CysZ family members are 28–30 kDa bacterial inner-membrane proteins found exclusively in prokaryotes with no apparent homology to any of the established channel or transporter folds, and are scarcely studied in the literature. The CysZ protomer is an alpha-helical integral membrane protein with two long transmembrane (TM) helices (H2b and H3a) and two pairs of shorter helices (H4b-H5a and H7-H8) that insert only partially into the membrane (hemi-penetrating), forming a funnel or tripod-like shape within the membrane. The protein has an extra-membranous hydrophilic ‘head’, comprising an iris-like arrangement of the two short helices, H1 and H6, and kinked helices H3b, H4a, and H5b. Besides not resembling other transporter structures, CysZ mediates sulfate flux into cells or proteoliposomes without coupling to ion gradients, partner proteins, or exogenous energy sources such as ATP.

The structure of PfCysZ was solved second, to 3.5 Å resolution, with crystals also belonging to space group C2. Although PfCysZ and IlCysZ share 42% sequence identity, molecular replacement failed to find a convincing solution, and we instead used SeMet-derivatized PfCysZ to obtain phase information by multi-crystal SeMet SAD. Unlike PdCysZ, both IlCysZ and PfCysZ crystallize as dimers, in agreement with their different behavior in detergent-containing solution. The PfCysZ dimer is also arranged in an antiparallel orientation but with a different dimer interface. In the PfCysZ structure, helices H4b-H5a together form a narrower angle with helices H2 and H3, and tuck-in closer to the rest of the molecule. The resulting dumbbell-shaped PfCysZ dimer is predicted, by OPM/PPM (Orientation of Proteins in Membranes), to lie in the membrane at a 31° tilt to the perpendicular, in agreement with the position of its central hydrophobic belt, as revealed by surface-electrostatics calculations. On the other hand, the PfCysZ dimer resembles the transverse pair of protomers lying at a tilt, just as was predicted by OPM, along the side of the PdCysZ hexamer when viewed from inside the plane of the membrane. Disulfide-trapping experiments of the transverse dimer, performed by crosslinking a pair of mutants (L161C-A164C) on helix H5 of PfCysZ, as well as the corresponding pair in IlCysZ (V157C-Q163C) confirm the dimer interface observed in the structures of PfCysZ and IlCysZ, and, as a consequence, the antiparallel assembly of the two proteins. The ‘transverse’ dimer structure of PfCysZ clarified the possibility for ion permeation by showing that openings in its two protomers aligned across the putative membrane; however, the prospective transduction pathway would then be open on one side to the bilayer. In the case of IlCysZ and PfCysZ, this assembly may have come apart into the subsequently crystallized dimeric components during the process of detergent extraction from the membrane and purification.

>[2x]MPAPVLSGPQYLREGLKLVLSPGLRLFVLLPLLINLVLFVGLIYFAGHQFSLWVDALMPSLPHWLSFLNYLLWPLFVVLVALMVFFTFTMLANIIAAPFNGFLSEKVEAVVRGVDNSPPFSWGELIAMVPRTLAREMRKLGYFLPRAIALLILSFIPVLNLVAAPLWLIFGVWMMAIQYIDYPADNHKLGWNEMLAWLREKRWQSLSFGGIVYLVLLIPVVNILMMPAAVAGATLFWVRERGDEALARTRA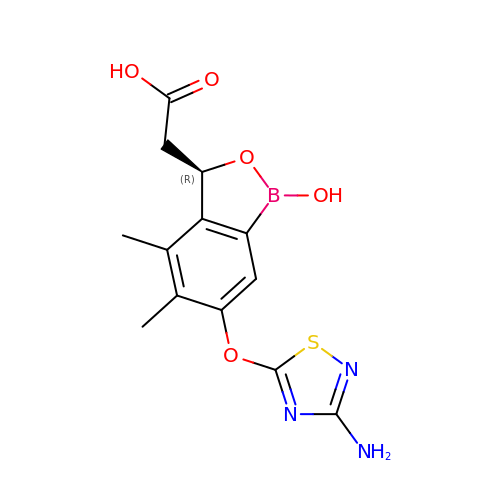{(3R)-6-[(3-amino-1,2,4-thiadiazol-5-yl)oxy]-1-hydroxy-4,5-dimethyl-1,3-dihydro-2,1-benzoxaborol-3-yl}acetic acid | C13 H14 B N3 O5 S | CXFHZAGALDYYDH-SECBINFHSA-N>QQASTLPDLAEQFAPPDVAPPLLIKLVEAIEKKGLECSTLYRTQSSSNPAELRQLLDCDTASLDLEMFDVHVLADAFKRYLLDLPNPVIPVAVSSELISLAPEVQSSEEYIQLLKKLIRSPSIPHQYWLTLQYLLKHFFKLSQTSSKNLLNARVLSELFSPLLFRFPAASSENTEHLIKIIEILISTEWNERQ[2x]

The N-terminal domains of p85α include an SH3 domain, capable of binding to proline-rich sequences, and a BH (breakpoint cluster region homology) domain. The BH domain can bind to and regulate several GTPases including Rab5, Rac1 and Cdc42. In addition, the p85α BH domain, either alone or together with the SH3 domain, can bind to and positively regulate PTEN activity. The p85α BH domain also exhibits Rab5 GAP activity to stimulate Rab5-mediated GTP hydrolysis required to inactivate Rab5-mediated protein trafficking functions.

We crystalized the wild type bovine p85α BH domain (105–319) and solved its structure to 2.25 Å resolution. X-ray diffraction data collection and structure refinement statistics for bovine p85α (105–319) wild type is provided in Supplementary Table S1. The BH domain dimers observed within the crystal structures are mediated by reciprocal interactions between M176 from one monomer fitting into a hydrophobic pocket created by L161, 177 (Ile in human, Phe in bovine), and V181 in the other monomer. The buried surface area in the bovine p85α BH–BH crystal lattice is 535 Å2, similar to in the human p85α BH–BH crystal lattice (527 Å2).>GICKSSDCIKSAARLIQNMDATTEPCTDFFKYACGGWLKRNVIPETSSRYGNFDILRDELEVVLKDVLQEPKTEDIVAVQKAKALYRSCINESAIDSRGGEPLLKLLPDIYGWPVATENWEQKYGASWTAEKAIAQLNSKYGKKVLINLFVGTDDKNSVNHVIHIDQPRLGLPSRDYYECTGIYKEACTAYVDFMISVARLIRQEERLPIDENQLALEMNKVMELEKEIANATAKPEDRNDPMLLYNKMTLAQIQNNFSLEINGKPFSWLNFTNEIMSTVNISITNEEDVVVYAPEYLTKLKPILTKYSARDLQNLMSWRFIMDLVSSLSRTYKESRNAFRKALYGTTSETATWRRCANYVNGNMENAVGRLYVEAAFAGESKHVVEDLIAQIREVFIQTLDDLTWMDAETKKRAEEKALAIKERIGYPDDIVSNDNKLNNEYLELNYKEDEYFENIIQNLKFSQSKQLKKLREKVDKDEWISGAAVVNAFYSSGRNQIVFPAGILQPPFFSAQQSNSLNYGGIGMVIGHEITHGFDDNGRNFNKDGDLVDWWTQQSASNFKEQSQCMVYQYGNFSWDLAGGQHLNGINTLGENIADNG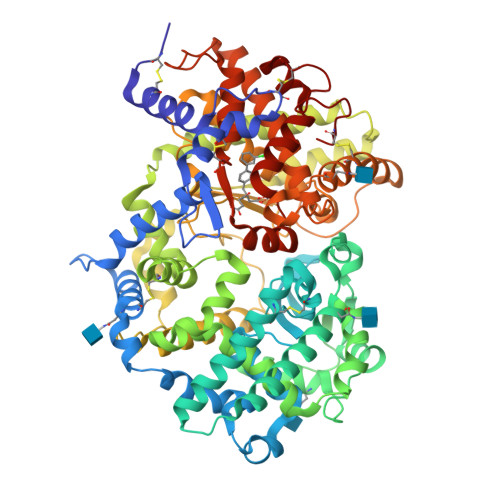GLGQAYRAYQNYIKKNGEEKLLPGLDLNHKQLFFLNFAQVWCGTYRPEYAVNSIKTDVHSPGNFRIIGTLQNSAEFSEAFHCRKNSYMNPEKKCRVW[2x]>[3x]MGSSIAPSLAVADLFNVNGLVAVVTGGATGIGLMMVRALEENGAKVYIVGRRKEVLEKVAKNEAKHGNIIPLQGDASSKDDLERIVAHITKETGYINLLVANAGIPGPAPIKMSPSSSLADIQKDLWNTDPAEFEHIFNVHVRGAYFSFAAFLPLLSAGNEKGNVPQSSQMIITGSIGAFGRVPLAHYAYSASKAGVTH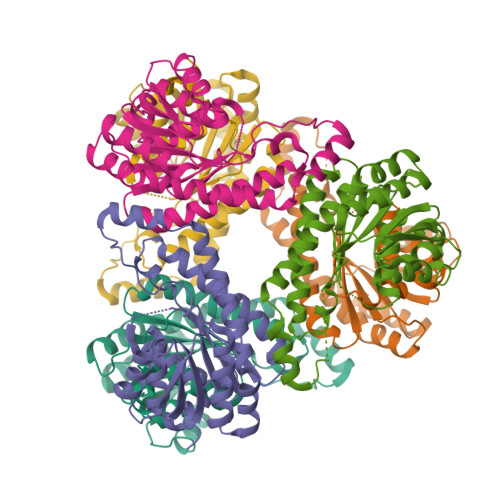MAKQLATAFTKYGIRFNVIAPGLYPSEMTEEIVKGTHQLTPDEYAMKVSPLGRPGNDEDVAGCILWLASKAGAWVSGNVLVTDGGKLGLVPSSY[(3R)-1-hydroxy-4,5-dimethyl-6-(pyrazin-2-yloxy)-1,3-dihydro-2,1-benzoxaborol-3-yl]acetic 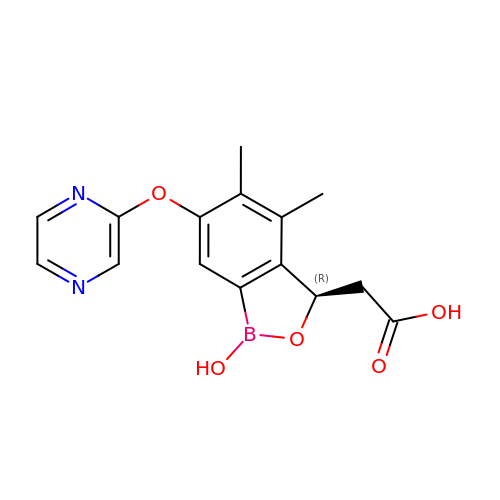acid | C15 H15 B N2 O5 | MTHDAYXINWUJNY-GFCCVEGCSA-N>[12x]AAEVLLLDSKAQQTELEWISSPPNGWEEISGLDENYTPIRTYQVCQVMEPNQNNWLRTNWISKGNAQRIFVELKFTLRDCNSLPGVLGTC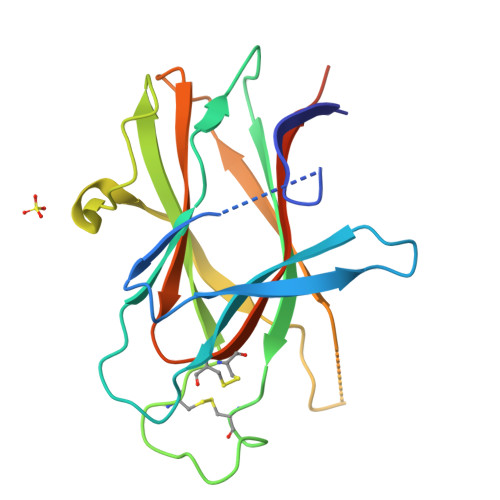KETFNLYYYETDYDTGRNIRENLYVKIDTIAADESFTQGDLGERKMKLNTEVREIGPLSKKGFYLAFQDVGACIALVSVKVYYKKEFVEHHHHHHHH> SSQIRQNYSTEVEAAVNRLVNLYLRASYTYLSLGFYFDRDDVA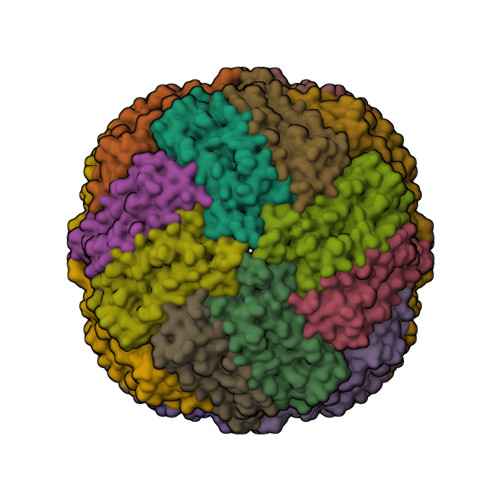LEGVCHFFRELAEEKREGAERLLKMQNQRGGRALFQDLQKPSQDEWGTTLDAMKAAIVLEKSLNQALLDLHALGSCQADPHLADFLESHFLDEEVKLIKKMGDHLTNIQRLVGSQAGLGEYLFERLTLKHD2-O-{4-[AMINO(IMINO)METHYL]PHENYL}-5-O-{3-[AMINO(IMINO)METHYL]PHENYL}-1,4:3,6-DIANHYDRO-D-GLUCITOL | 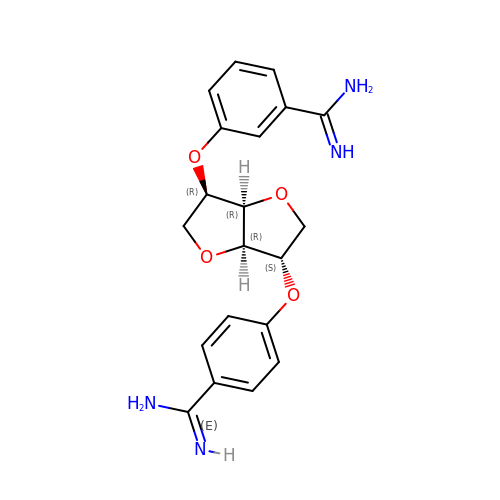C20 H22 N4 O4 | DKBAWRNTUZFJKV-BSDSXHPESA-N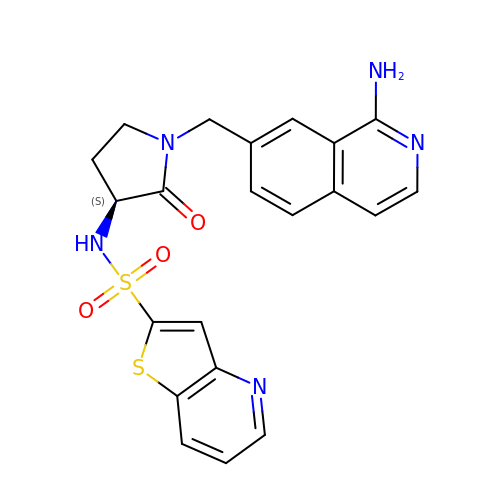THIENO[3,2-B]PYRIDINE-2-SULFONIC ACID [1-(1-AMINO-ISOQUINOLIN-7-YLMETHYL)-2-OXO-PYRROLDIN-3-YL]-AMIDE | C21 H19 N5 O3 S2 | NVKDOURNRJCKJE-INIZCTEOSA-N> MGSSHHHHHHSQDPMNRPSFNEAWLAFRKVNHSVADVGSIIGGNVGKNITGGYFQNACPIRMSYVLNATGFPIARNSPYAKVSGADNKFYIYRVNDMIDYLTHTMGKPDLIVNNPKQSDFIGKKGIIVVKGHGWSNARGHVTLWNGSICSDQC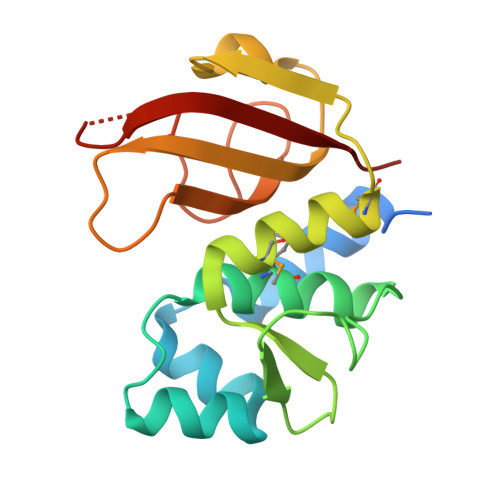HLLNDPDNGPFVPEVGTLWILP>DLLAGGKDDVKATFGADSFVMMCIIIAELIVGVAMYIRTKNLLILLGLVVVIVFTTVG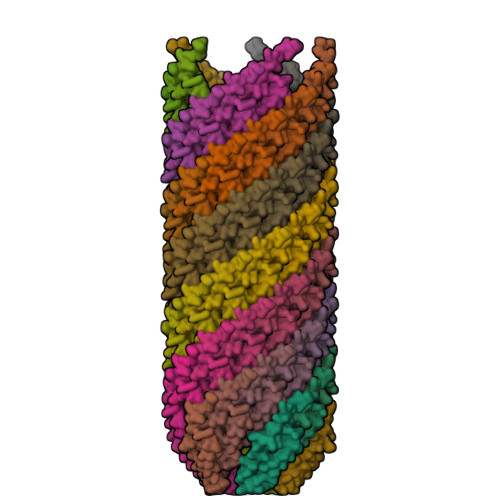LTFIK[80x]> MSDILQELLRVSEKAANIARACRQQETLFQLLIEEKKEGEKNKKFAVDFKTLADVLVQEVIKENMENKFPGLGKKIFGEESNELTNDLGEKIIMRLGPTEEETVALLSKVLNGNKLASEALAKVVHQDVFFSDPALDSVEINIPQDILGIWVDPIDSTYQYIKGSADITPNQGIFPSGLQCVTVLIGVYDIQTGVPLMGVINQPFVSQDLHTRRWKGQCYWGLSYLGTNIHSLLP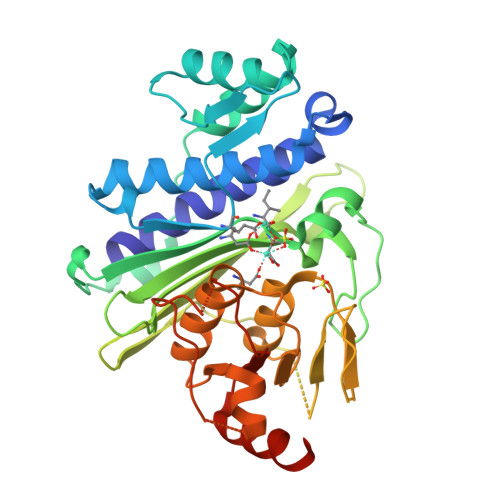PVSTRSNSEAQSQGTQNPSSEGSCRFSVVISTSEKETIKGALSHVCGERIFRAAGAGYKSLCVILGLADIYIFSEDTTFKWDSCAAHAILRAMGGGMVDLKECLERNPDTGLDLPQLVYHVGNEGAAGVDQWANKGGLIAYRSEKQLETFLSRLLQHLAPVATHT>IARPTLEAHDYDREALWSKWDNASDSQRRLAEKWLPAVQAADEMLNQGISTKTAFATVAGHYQVSASTLRDKYYQVQKFAKPDWAAALVDGRGASRRNVHKSEFDEDAWQFLIADYLRPEKPAFRKCYERLELAAREHGWSIPSRATAFRRIQQLDEAMVVACREGEHALMHLIPAQQRTVEHLDAMQWINGDGYLHNVFVRWFNGDVIRPKTWFWQDVKTRKILGWRCDVSENIDSIRLSFMDVVTRYGIPEDFHITIDNTRGAANKWLTGGAPNRYRFKVKEDDPKGLFLLMGAKMHWTSVVAGKGWGQAKPVERAFGVGGLEEYVDKHPALAGAYTGPNPQAKPDNYGDRAVDAELFLKTLAEGVAMFNARTGRETEMCGGKLSFDDVFEREYARTIVRKPTEEQKRM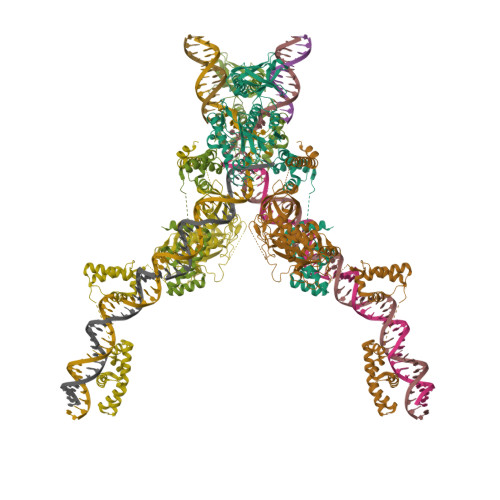LLLPAEAVNVSRKGEFTLKVGGSLKGAKNVYYNLALMLAGVKKVVVRFDPQQLHSTVYCYTLDGRFICEAECLAPVAFNDAAAGREYRRRQKQLKSATKAAIKAQKQMDALEVAELLP[2x]>IASQLLTLSAPAEAAVKTNVGPSPSRAGVGYDVIVIGGGFAGVTAAREASRSGLKTLILEGRSRLGGRTFTSKLQNQKVELGGTWVHWTQPNVWTEIMHYGLEVEETVGLANPETVIWVTEDNVKRAPAAEAFEIFGSACNEYYKEARNIYPRPFEPFFERKKLQHVDGLSAADYLEKLPLTREQKDMMDSWLSGNGHNYPETIAYSEIMRWFALSNFNMPTMFDSI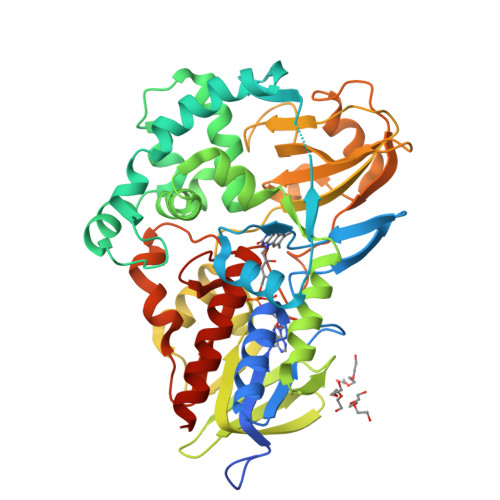ARYKIKTGTHSLLEAIMADGNSEVKLSTPVTKVNQDKDKVTVTTEDGVFTASAVIVAVPINTLHDIEYSPKLSAAKVDMGSQRHAGAGVKGYIRVAQNVGNVMTYAPARNKLTPFTSVFTDHVDEAGTLLIAFSADPKLIDINDIKAVEKALQPLLPGVEVTASYGYDWNLDPFSKGTWCTYRPNQTTRYLTELQKREGRLFFAGSDMANGWRGFIDGAIENGREVGHQVATYLKRENDNAHHHHHH[2x]> GHHHHHHEFDQVQYENTLKNFKIREQQFDNSWAAGFSMAALLNATKNTDTYNAHDIMRTLYPEVSEQDLPNCATFPNQMIEYGKSQGRDIHYQEGVPSYNQVDQLTKDNVGIMILAQSVSQNPNDPHLGHALAVVGNAKINDQEKLIYWNPWDTELSIQDADS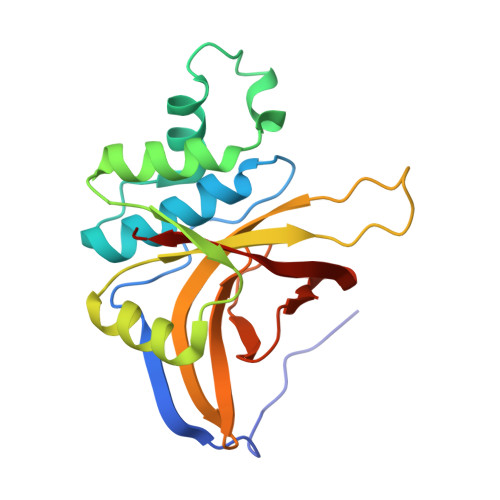SLLHLSFNRDYNWYGSMIGY>SKPFTVPILTVEEMSNSRFPIPLEKLYTGPSSAFVVQPQNGRCTTDGVLLGTTQLSAVNICNFRGDVTRVGISHDYTMNLVSQNWNNYDPTEEIPAPLGTPDFVGKIQGLLTQTTRADGSTRAHKATVSTGSVHFTPKLGSVQFTTDTNNDFQTGQNTKFTPVGVIQDGDHHQN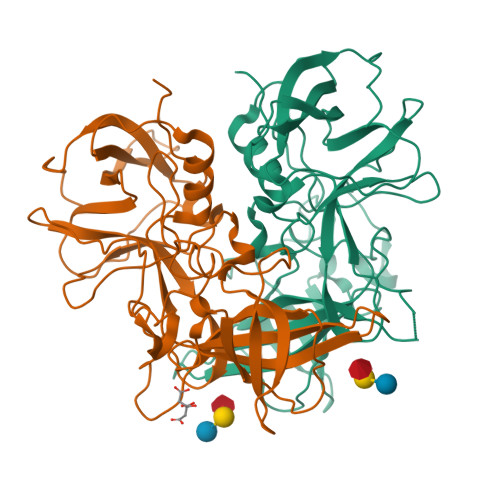EPQQWVLPNYSGTSGHNVHLAPAVAPTFPGEQLLFFRSTMPGCSGYPNMNLDCLLPQEWVSHFYQEAAPAQSDVALLRFVNPDTGRVLFECKLHKSGYITVAHTGPYDLVIPPNGYFRFDSWVNQFYTLAPM[2x]>MAIKVGINGFGRIGRSFFRASWGREEIEIVAINDLTDAKHLAHLLKYDSVHGIFKGSVEAKDDSIVVDGKEIKVFAQKDPSQIPWGDLGVDVVIEATGVFRDRENASKHLQGGAKKVIITAPAKNPDIT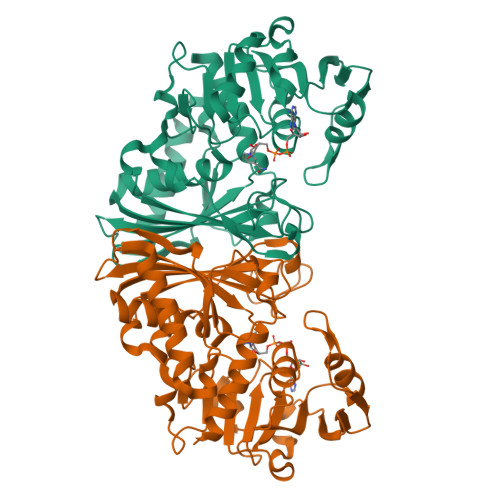VVLGVNEEKYNPKEHNIISNASCTTNCLAPCVKVLNEAFGVEKGYMVTVHAYTNDQRLLDLPHKDFRRARAAAINIVPTTTGAAKAIGEVIPELKGKLDGTARRVPVPDGSLIDLTVVVNKAPSSVEEVNEKFREAAQKYRESGKVYLKEILQYCEDPIVSTDIVGNPHSAIFDAPLTQVIDNLVHIAAWYDNEWGYSCRLRDLVIYLAERGL[2x]>MAGFLKVVQLLAKYGSKAVQWAWANKGKILDWLNAGQAIDWVVSKI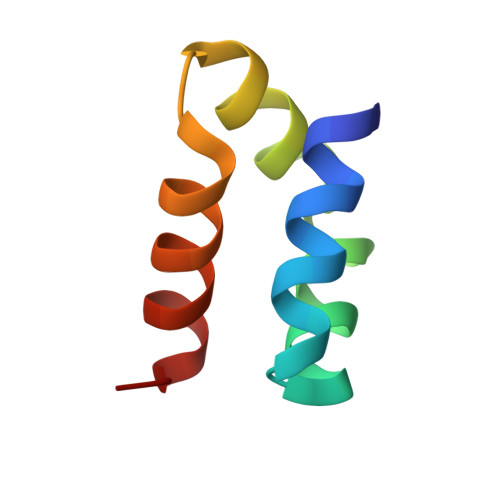KQILGIK[4x]N-hydroxy-4-({[(pyridin-3-yl)methyl][(2,3,4,5-tetrafluorophenyl)sulfonyl]amino}methyl)benzamide 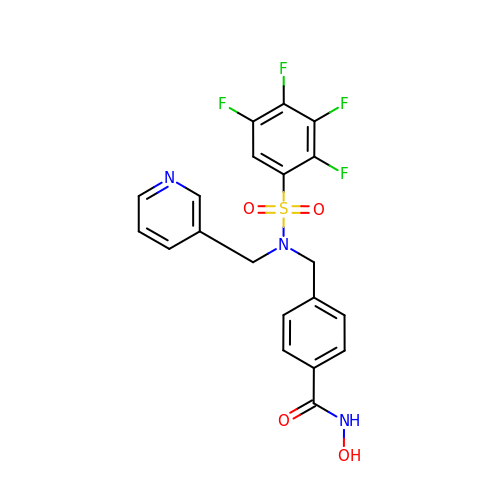| C20 H15 F4 N3 O4 S | HBOMISXRZUHCSH-UHFFFAOYSA-N> GHMGHMSGSNTEEEIRMELSPDLISACLALEKYLDNPNALTERELKVAYTTVLQEWLRLACRSDAHPELVRRHL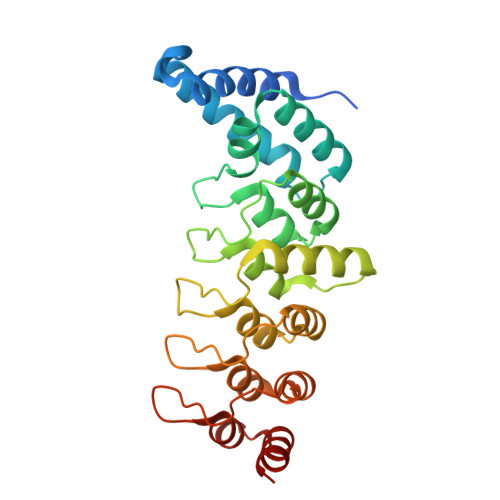VTFRAMSARLLDYVVNIADSNGNTALHYSVSHANFPVVQQLLDSGVCKVDKQNRAGYSPIMLTALATLKTQDDIETVLQLFRLGNINAKASQAGQTALMLAVSHGRVDVVKALLACEADVNVQDDDGSTALMCACEHGHKEIAGLLLAVPSCDISLTDRDGSTALMVALDAGQSEIASMLYSRMNIK>MNPYIYLGGAILAEVIGTTLMKFSEGFTRLWPSVGTIICYCASFWLLAQTLAYIPTGIAYAIWSGVGIVLIS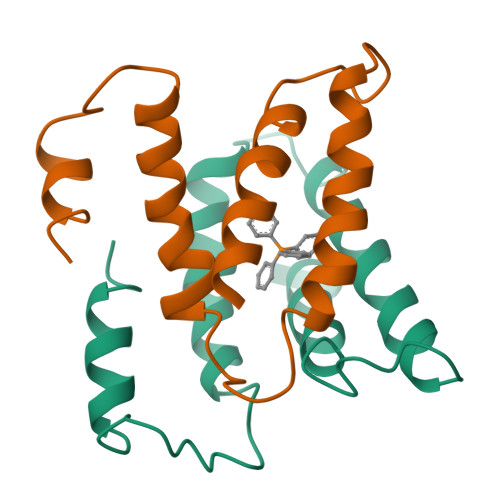LLSWGFFGQRLDLPAIIGMMLICAGVLIINLLSRSTPH[4x]>FQGAMGSRVVILFTDIEESTALNERIGDRAWVKLISSHDKLVSDLVRRQSGHVVKSQGDGFMVAFARPEQAVRCGIELQRALRRNANRKRHEEIRVRIGIH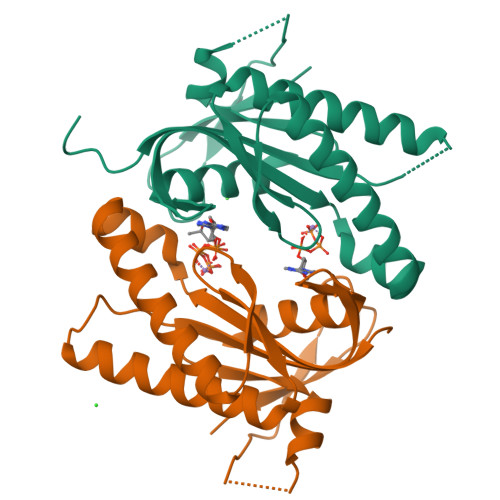MGRSVRRGDDLFGRNVAMAARVAAQAAGGEILVSQPVRDALSRSDGIRFDDGREVELKGFSGTYRLFAVL[2x]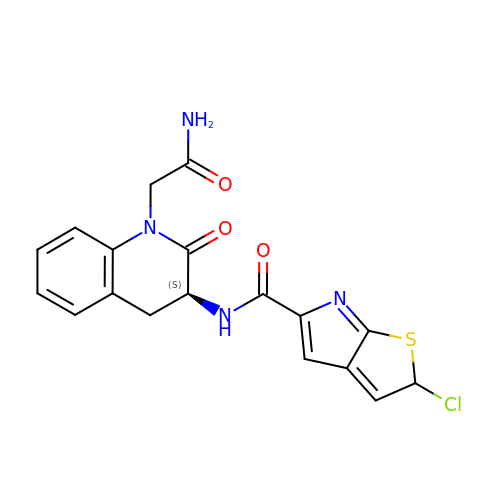(2S)-N-[(3S)-1-(2-AMINO-2-OXOETHYL)-2-OXO-1,2,3,4-TETRAHYDROQUINOLIN-3-YL]-2-CHLORO-2H-THIENO[2,3-B]PYRROLE-5-CARBOXAMIDE | C18 H15 Cl N4 O3 S | ACSGSLPOHKRZCY-GXTWGEPZSA-N>MYYFIPSWSGSGKRVWHRDIIPWYRSMQRLEFDDTIHQIRIFHSENLPVKLLLQAYMPHARYFLHRQDIFETEYYSVFDEIQAVESNDMQVLQIKDLEWEDDCEFIYTPFLIIVRRQGQLYAHVEFGVEGFISFIKFFKDDQLEKLNIFDDRGFVSSIVYYEDGQEVCQDYLNPNGDWRIREYLKFENSHVVVNPVFSRDFDKLEYECMPDLILEKLGYYISHNVEEDSRFVVAAQPFTNQGVLDLLPQHSHSILSFFHERNQASNIENLKADLEYADLVLTDRMDFKETLQNYFPLQAEKIHYLSPFDTRLQLGKSQQRHESKIFYQIDLSELLNDYAIFKVLFYVAQHPDTELVIGVYNAWQEGIKQVENKVEELISDYLDLKDFIKKSFKNNQAENPLPENQELEYRFRIRNITDELSL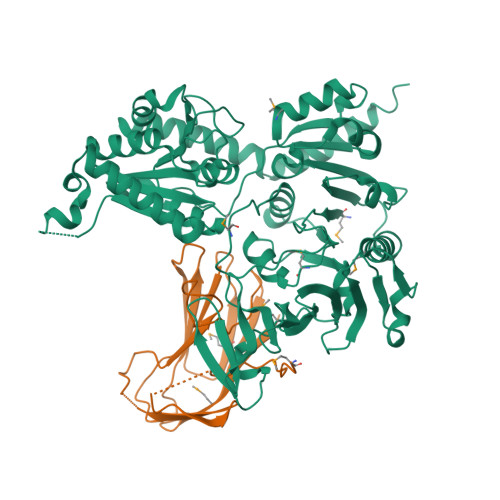IQELDDTRLIIDLSQQPNLYTQIAGISAGIPQINLVASDYVTHLQNGYILDSISQLAVAADYYLQGLKNWNQALIYSIEKIKLNTGHQVIKRWEKWLKEAIDEKVDKLVPR[4x];>[4x]MKIQKHKEIYWGELRGASISKTRKDFTYLYGSTIIFHSPDQVYFENKLIASGQTIHEWSSSWNYQGDRQVPSLPLLKRGRSYSLTRDMTSYPSESVFLKLIFFDRYNREVSNHVERSDKMTFTYPEEAYSYKVQLLSAGVESFEFHCLRIEEILEESNG>[2x]MPNIKIFSGSSHQDLSQKIADRLGLELGKVVTKKFSNQETCVEIGESVRGEDVYIVQSGCGEINNNLMELLIMINACKIASASRVTAVIPCFPYA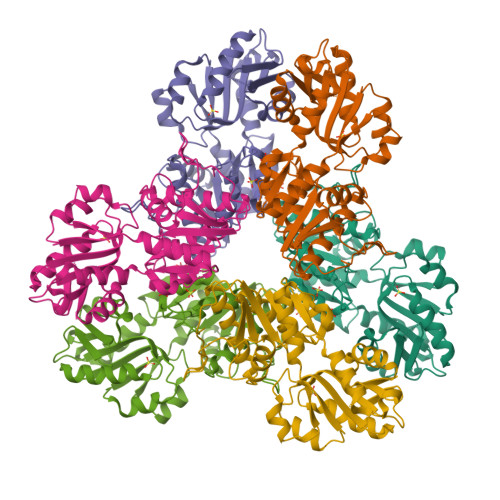RQDKKDKSRAPISAKLVANMLSVAGADHIITMDLHASQIQGFFDIPVDNLYAEPAVLKWIRENISEWRNCTIVSPDAGGAKRVTSIADRLNVDFALIHKERKKANEVDRMVLVGDVKDRVAILVDDMADTCGTICHAADKLLSAGATRVYAILTHGIFSGPAISRINNACFEAVVVTNTIPQEDKMKHCSKIQVIDISMILAEAIRRTHNGESVSYLFSHVPLLEHHHHHH>[7x]MHHH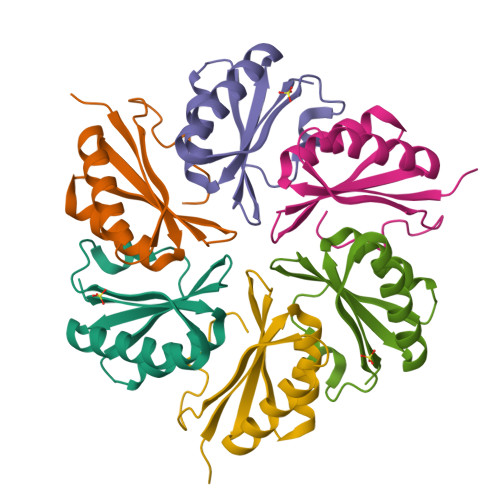HHHQQEALGMVETKGLTAAIEAADAMVASANVMLVGYEKIGGSGGLVTVIVRGDVGAVKAATDAGAAAARNVGEVKAVHVIPRPHTDVEKILPKGISQ>HHHHHHFNLPPGNYKKPVLLYASNGGHFLRILPDGTVDGTRDRSDQHIQLQLSAESVGEVYIKSTETGQYLAMDTDGLLYGSQTPNEECLFLERLEENHYNTYISKKHAEKNWFVGLKKNGSVKRGPRTHYGQKAI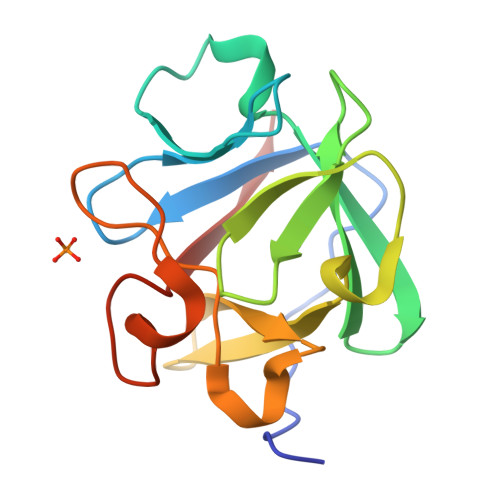LFLVLPVSSD[2x]> GGAAACGTT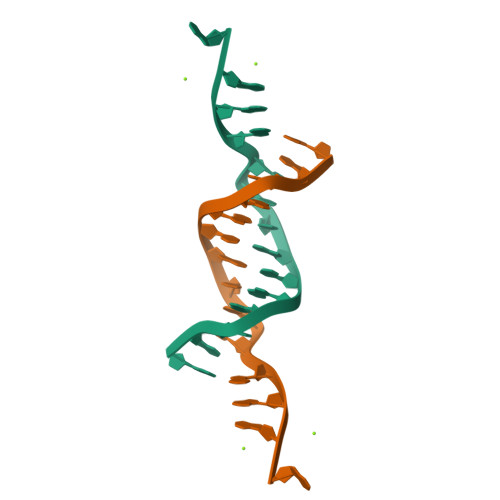GGAGA> MAGAIASRMSFSSLKRKQPKTFTVRIVTMDAEMEFNCEMKWKGKDLFDLVCRTLGLRETWFFGLQYTIKDTVAWLKMDKKVLDHDVSKEEPVTFHFLAKFYPENAEEELVQEITQHLFFLQVKKQILDEKIYCPPEASVLLASYAVQAKYGDYDPSVHKRGFLAQEELLPKRVINLYQMTPEMWEERITVWYAEHRGRARDEAEMEYLKIAQDLEMYGVNYFAIRNKK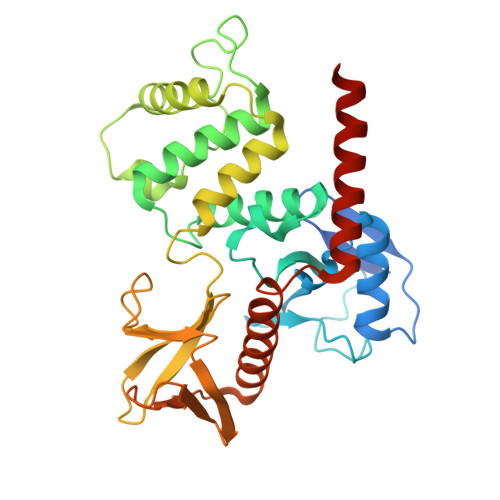GTELLLGVDALGLHIYDPENRLTPKISFPWNEIRNISYSDKEFTIKPLDKKIDVFKFNSSKLRVNKLILQLCIENHDLFMRRRKADSLEVQQMKAQAREEKARKQMERQRL> GPGSMVECITPEAIFIGANKQTQVSDIHKVKKIVAFGAGKTIALWDPIEPNNKGVYATLKGHEAEVTCVRFVPDSDFMVSASEDHHVKIWKFTDYSHLQCIQTIQHYSKTIVALSALPSLISVGCADGTISIWRQNIQNDEFGLAHEFTIKKGFFYPLCLSLSKVEEKKYLLAIGGTNVNVFIASFILSDSGIEKCRVVAELEGHEDWVKSLAFRHQETPGDYLLCSGSQDRYIRLWRIRINDLIDDSEEDSKKLTLLSNKQYKFQIDDELRVGINFEALIMGHDDWISSLQWHESRLQLLAATADTSLMVWEPDETSGIWVCSLRLGEMSSKGASTATGSSGGFWSCLWFTHERMDFFLTNGKTGSWRMWATKDNIICDQRLGISGATKDVTDIAWSPSGEYLLATSLDQTTRLFAPWIYDASGRKREIATWHEFSRPQIHGYDMIC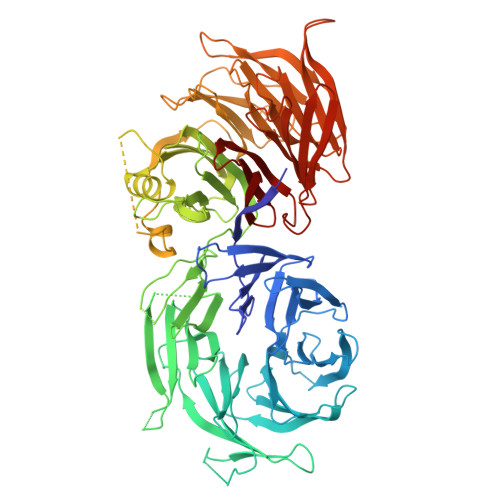VETVTDTRFVSGGDEKILRSFDLPKGVAGMLQKFVGIQFEEKSEMPDSATVPVLGLSNKAGEDDANEDDEEEEGGNKETPDITDPLSLLECPPMEDQLQRHLLWPEVEKLYGHGFEITCLDISPDQKLIASACRSNNVQNAVIRIFSTENWLEIKPALPFHSLTITRLKFSKDGKFLLSVCRDRKWALWERNMEDNTFELRFKNEKPHTRIIWDADWAPLEFGNVFVTASRDKTVKVWRHQKEPADDYVLEASIKHTKAVTAISIHDSMIREKILISVGLENGEIYLYSYTLGKFELITQLNEDITPADKITRLRWSHLKRNGKLFLGVGSSDLSTRIYSLAYE5-METHYL-8-(1H-PYRROL-2-YL)[1,2,4]TRIAZOLO[4,3-A]QUINOLIN-1(2H)-ONE | C15 H12 N4 O | 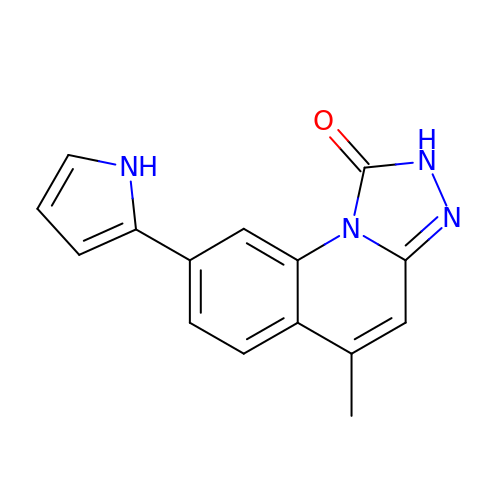XHMYMTXQNURDOQ-UHFFFAOYSA-N> MSAKLISVTKPV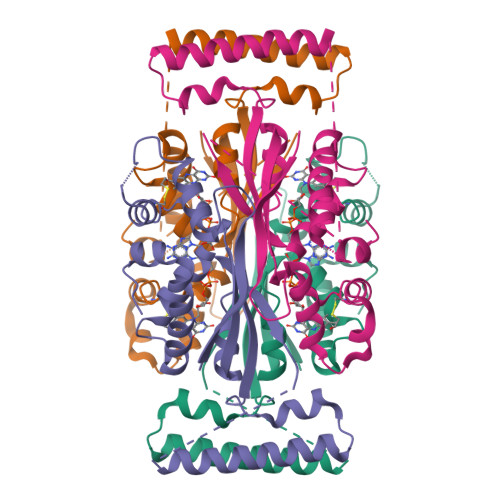VEGVNTAEELIAYAARVSNPENQINNKTASGLLKYCIRHKHWSIFETAFMTLELKTSRGIAAQVLRHRSFHFQEFSQRYASVMETPPPHQARFQDHKNRQNSLDTVPEDDQTWWATEQEKLYAQSMELYNKALEKGIAKECARFILPLSTPTTIYMSGTIRDWIHYIELRTSNGTQREHIDLANACKEIFIKEFPSIAKALDWVH;> MSAKLISVTKPVVEGVNTAEELIAYAARVSNPENQINNKTASGLLKYCIRHKHWSIFETAFMTLELKTSRGIAAQVIRHRSFHFQEFSQRYASVMETPPPHQARFQDHKNRQNSLDTVPEDDQTWWATEQEKLYAQSMELYNKALEKGIAKECARFILPLSTPTTIYMSGTIRDWIHYIELRTSNGTQREHIDLANACKEIFIKEFPSIAKALDWVH> HHHHHHGSMQSIKSNESFKSVINSDTPVIVKFEAGWCPDCRAMDLWIDPIVEQYNDYQWYTV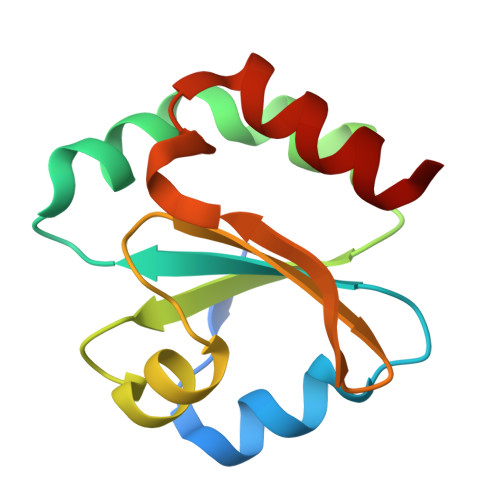NRDELEDVVVENEVMGIPSLLVFKNGDKIAHLHSANAKSPEQVESFLAETFK> MEFFGESWKKHLSGEFGKPYFIKLMGFVAEERKHYTVYPPPHQVFTWTQMCDIKDVKVVILGQNPYHGPNQAHGLCFSVQRPVPPPPSLENIYKELSTDIEDFVHPGHGDLSGWAKQGVLLLNAVLTVRAHQANSHKERGWEQFTDAVVSWLNQNSNGLVFLLWGSYAQKKGSAIDRKRHHVLQTAHPS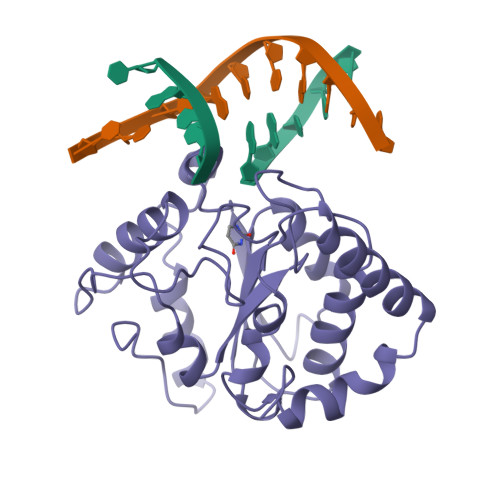PRSVYRGFFGCRHFSKTNELLQKSGKKPIDWKEL> MYNGKDRAQNSYQPMYQRPMQVQGQQQAQSFVGKKNTIGSVHGKAPMLMANNDVFTIGPYRARKDRMRVSVLEKYEVIGYIAAGTYGKVYKAKRQINSGTNSANGSSLNGTNAKIPQFDSTQPKSSSSMDMQANTNALRRNLLKDEGVTPGRIRTTREDVSPHYNSQKQTLIKKPLTVFYAIKKFKTEKDGVEQLHYTGISQSACREMALCRELHNKHLTTLVEIFLERKCVHMVYEYAEHDLLQIIHFHSHPEKRMIPPRMVRSIMWQLLDGVSYLHQNWVLHRDLKPANIMVTIDGCVKIGDLGLARKFHNMLQTLYTGDKVVVTIWYRAPELLLGARHYTPAVDLWSVGCIFAELIGLQPIFKGEEAKLDSKKTVPFQVNQLQRILEVLGTPDQKIWPYLEKYPEYDQITKFPKYRDNLATWYHSAGGRDKHALSLLYHLLNYDPIKRIDAFNALEHKYFTESDIPVSENVFEGLTYKYPARRIHTNDNDIMNLGSRTKNNTQASGITAGAAANALGGLGVNRRILAAAAAAAAAVSGNNASDEPSRKKNRR;> MSGSFWTSTQRHHWQYTKASLAKERQKLWLLECQLFPQGLNIVMDSKQNGIEQSITKNIPITHRDLHYDKDYNLRIYCYFLIMKLGRRLNIRQYALATAHIYLSRFLIKASVREINLYMLVTTCVYLACKVEECPQYIRTLVSEARTLWPEFIPPDPTKVTEFEFYLLEELESYLIVHHPYQSLKQIVQVLKQPPFQITLSSDDLQNCWSLINDSYINDVHLLYPPHIIAVACLFITISIHGKPTKGSSLASAASEAIRDPKNSSSPVQIAFNRFMAESLVDLEEVMDTIQEQITLYDHWDKYHEQWIKFLLHTLYLRPASAI;> MNNGSGRYLLTPPDDLHPYVPSSKPQEQVYPDFKPWEHTAAEDQILANFVAKGFYHTPMVNFESISARSSVHESLVTQSNILSQQFDKIIKIREDHINKIPSNSTTTLHGPGFQLPNRITLTDHRKETWLHELSSSHTSLVKIGKFIPHGLKRRQVIEQCYLKFIPLKRAIWLIKCCYFIEWKSNHKKKRSNAAGADDAISMHLLKDWTDTFVYILEKLIFDMTNHYNDSQQLRTWKRQISYFLKLLGNCYSLRLINKEIFHHWLVEFINKMENFEFLPLSLHILMIFWNDICQIDTNAPVAATITSSQKEPFFLVTKITDMLLHKYYIVSSSKSMINDENYIINDIKKNNKIKLNILKILSSLILKIFQEQSLEVFIFPTSNWEIYKPLLFEIVSNADTNQNSDMKKKLELISYRNESLKNNSSIRNVIMSASNANDFQLTIVTCKQFPKLSCIQLNCIDTQFTKLLDDNPTEFDWPTYVDQNPLTMHKIIQLILWSIHPSRQFDHYESNQLVAKLLLLRINSTDEDLHEFQIEDAIWSLVFQLAKNFSAQKRVVSYMMPSLYRLLNILITYGIIKVPTYIRKLISSGLLYLQDSNDKFVHVQLLINLKISPLMKSQYNMVLRNVMEYDVKFYEIFNFDQLVEITEQIKMRILSNDITNLQLSKTPLSIKIMVAEWYLSHLCSGILSSVNRTVLLKIFKIFCIDLEVFHHFFKWIEFIVYHQLLSDIESLEALMDILLCYQKLFSQFINDHILFTKTFIFIYKKVLKEKDVPAYNVTSFMPFWKFFMKNFPFVLKVDNDLRIELQSVYNDEKLKTEKLKNDKSEVLKVYSMINNSNQAVGQTWNFPEVFQVNIRFLLHNSEIIDTNTSKQFQKARNNVMLLIATNLKEYNKFMSIFLKRKDFTNKNLIQLISLKLLTFEVTQNVLGLEYIIRLLPINLENNDGSYGLFLKYHKEQFIKSNFEKILLTCYELEKKYHGNECEINYYEILLKILITYGSSPKLLATSTKIIMLLLNDSVENSSNILEDILYYSTCPSETDLNDIPLGSGQPDNDTVVTNDDKSDDDDHTVDEIDHVEYYVMMDFANLWVFQAFTCFCIKKIMENNEPAMAMEDLKNFIFQIIEITNSNDLCSQIFDQLKDMQTIEMITQIVEKDFCTSCLQNNNQKIDDNYIVVVIEIITSLSMRFQRETSGMIVISMENYHLLIKIIRQLSELNEGNLSKREIQIDAVLKIFSFHQDSIFQRIIADLSADKPTSPFIDSICKLFDKISFNLRLKLFLYEILSSLKSFAIYSSTIDAPAFHTSGKVELPKKLLNLPPFQVSSFVKETKLHSGDYGEEEDADQEESFSLNLGIGIVEIAHENEQKWLIYDKKDHKYVCTFSMEPYHFISNYNTKYTDDMATGSNDTTAFNDSCVNLSLFDARFERKNPH;> MSSDASTYRLEDVLSSFYRVEKIKKINYHQYISKAQNDQWSIQMEFMLRKQDPKTLVALLSRDLWCFSINDDPVPTPPAIEHKPVSPDKIGTFTADYSKPNLPPHYALFLKALRRKIYINLALGSHNKLIQFGNACISLSGVPNYLVQLEPHLFVNGDLTVSLCAKNMGLVPMKEENLEESFLSKHALYLAPSGIRMHLAPASKQGYLITPPKHTELLLTTLSVSHGINLQNKKNLKWVAVVPDLGHLNGHTPTIASYLTPLLEAKKLVWPLHLIFAQPVADIENSTSGDPSEFHCLQDALDAIDDFIQLKQTAAYRTPGSSGVLSSNIAGTNPLSSDGAYTEQFQHYKNNSISSQPASYHSVQETNKISPKDFSPNFTGIDKLMLSPSDQFAPAFLNTPNNNINENELFNDRKQTTVSNDLENSPLKTELEANGRSLEKVNNSVSKTGSVDTLHNKEGTLEQREQNENLPSDKSDSMVDKELFGEDEDEDLFGDSNKSNSTNESNKSISDEITEDMFEMSDEEENNNNKSINKNNKEMHTDLGKDIPFFPSSEKPNIRTMSGTTKRLNGKRKYLDIPIDEMTLPTSPLYMDPGAPLPVETPRDRRKSVFAPLNFNPIIENNVDNKYKSGGKFSFSPLQKEEALNFDISMADLSSSEEEEDEEENGSSDEDLKSLNVRDDMKPSDNISTNTNIHEPQYINYSSIPSLQDSIIKQENFNSVNDANITSNKEGFNSIWKIPQNDIPQTESPLKTVDSSIQPIESNIKMTLEDNNVTSNPSEFTPNMVNSEISNLPKDKSGIPEFTPADPNLSFESSSSLPFLLRHMPLASIPDIFITPTPVVTISEKEQDILDLIAEQVVTDYNILGNLGIPKIAYRGVKDCQEGLITTTMLQLFSTFDRLNGNDTISKFYNMKQPYVFVKKHHELIKVKHDSQPFIKFLNFRPPNGIKNFKSLLLSSSFKEDCLSFAPTLSQTYINQELGFCELLKLTNEDPPGLMYLKAFDKNKLLLLAAQIVSYCSNNKNSIKNVPPILIILPLDNATLTELVDKANIFQVIKNEVC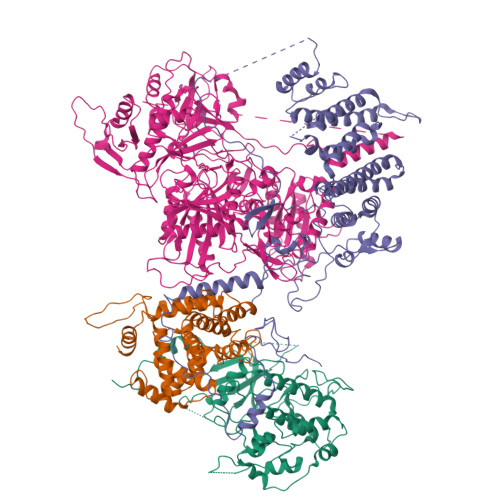AKMPNIELYLKVIPMDFIRNVLVTVDQYVNVAISIYNMLPPKSVKFTHIAHTLPEKVNFRTMQQQQMQQQQQQQQQQQNNSTGSSSIIYYDSYIHLAYSRSVDKEWVFAALSDSYGQGSMTKTWYVGNSRGKFDDACNQIWNIALNLASKKFGKICLILTRLNGILPDDELMNWRRLSGRNIHLAVVCVDDNSKISFIDEDKLYPSFKPIYKDTRFGGRMDMTRLYDYEIRDIDQDIHGIVFQHPFPLAHSQHRCAIRSGALIKFKKCDGDTVWDKFAVNLLNCPHSDSTQLLETILEEFRNLAALNVWYGLSDGEDGHIPWHILAVKKMMNTLVHTRVKIANTSAATVHTATSSSIILSDK The liver X receptors (LXRs) alpha (LXRα, NR1H3) and beta (LXRβ, NR1H2) are members of the nuclear hormone receptor (NHR) superfamily of transcription factors that function as heterodimers with the retinoid X receptor (RXR) and activate or repress gene expression in response to binding of cholesterol derivatives or synthetic ligands. Transcriptional responses of LXRs are known to directly result from ligand-induced conformational changes in the receptor: similarly to other NHRs, in the absence of ligands or in the presence of antagonists, LXRs form complexes with corepressors, while binding of agonist ligands forces the C-terminal helix H12 of the receptor to fold into the active state that creates an activation function-2 (AF-2) coactivator-binding surface. Reaching isoform selectivity by rational structure-based drug design has proven to be difficult since the ligand-binding pockets (LBPs) of LXRα and LXRβ are virtually identical. Since the adverse lipogenic effects are considered to be largely driven by LXRα23,28, drug discovery efforts have focused on developing LXRβ-selective compounds.

We have also included compounds AZ7–9 representing a structurally related series where the central scaffold ring is replaced by a maleimide core. AZ6 and compounds with higher potencies were assigned to the first class of ligands (high ABCA1 inducers, ED50 ≤ 11.3 µmol kg−1), while compounds AZ5, AZ8, AZ9, and LXR-623 with weaker potencies were assigned to the second class (low ABCA1 inducers). As no trends toward increased TG levels were observed for compounds AZ6–9 and LXR-623 within the explored concentration range, these ligands were assigned to a “non-lipogenic” class together with GW3965 (C2 = 40.2 µM) and BMS-852927 (C2 = 477 µM). Interestingly, the corresponding region of H3 in LXRα displayed a much broader range of ligand-dependent protection after 600 s: from 60% in BMS-852927 complex to no effect in the case of compounds LXR-623, AZ5, AZ8, and AZ9. Analysis of crystal structures of LXRβ LBD in complex with WAY-254011, AZ3, AZ6, and AZ8, as well as of previously published crystal structures of LXRβ31,40,55 reveals that GW3965 and BMS-852927 are the only compounds not forming a direct hydrogen bond with LXRβ His435 and therefore they do not stabilize the His435–Trp457 activation switch crucial for the agonistic conformation of H12. Other agonists form shorter hydrogen bonds of 2.5–3.1 Å essential for proper position of H12, which correlates with their activities both in LXRβ HDX-MS and functional assays.

> GVQLTAAQELMIQQLVAAQLQCNKRSFSDQPKVTPWPLGADPQSRDARQQRFAHFTELAIISVQEIVDFAKQVPGFLQLGREDQIALLKASTIEIMLLETARRYNHETECITFLKDFTYSKDDFHRAGLQVEFINPIFEFSRAMRRLGLDDAEYALLIAINIFSADRPNVQEPGRVEALQQPYVEALLSYTRIKRPQDQLRFPRMLMKLVSLRTLSSVHSEQVFALRLQDKKLPPLLSEIWDVHE> MRSLRTNYIYVLFKTTGLLFLLLLSACNRSGYIPENEVPKLPCRVDGACDATIIKMMTDLNKKGIKVASVGQNYLISIPASALFADQSPRLNWASYSLLNEIAAFLKQFRKIAITVTSYSSKYVSVKRERALTLARSRVVSEYLWSQGVDSRIIFTQGLGSDKPITSYTLGGDRSPNARVEITFRR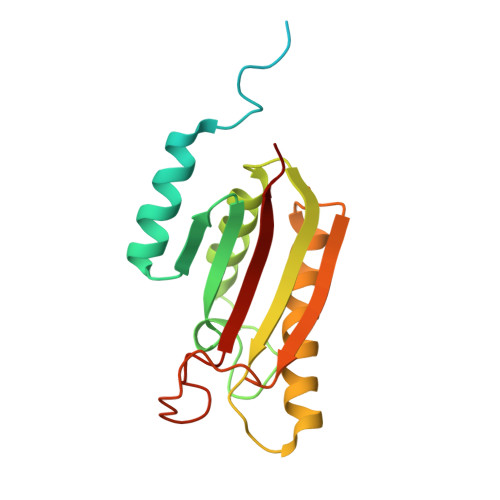AVA> MSEIGTGFPFDPHYVEVLGERMH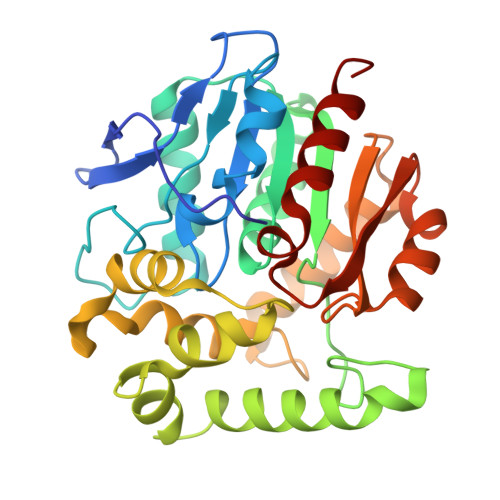YVDVGPRDGTPVLFLHGNPTSSYLWRNIIPHVAPSHRCIAPDLIGMGKSDKPDLDYFFDDHVRYLDAFIEALGLEEVVLVIHDWGSALGFHWAKRNPERVKGIACMEFIRPIPTWDEFHHTEVAEEQDHAEAARETFQAFRTADVGRELIIDQNAFIERVLPGGVVRPLTEVEMDHYREPFLKPVDREPLWRFPNELPIAGEPANIVALVEAYMNWLHQSPVPKLLFWGTPGALIPPAEAARLAESLPNCKTVDIGPGLHYLQEDNPDLIGSEIARWLPAL>SANLPTVLVTGASGRTGQIVYKKLKEGSDKFVAKGLVRSAQGKEKIGGEADVFIGDITDADSINPAFQGIDA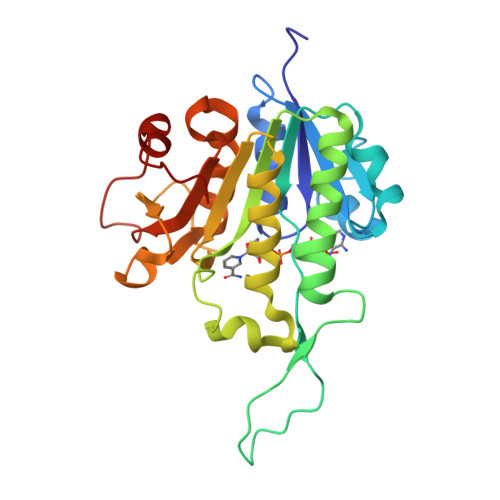LVILTSAVPKMKPGFDPTKGGRPEFIFEDGQYPEQVDWIGQKNQIDAAKVAGVKHIVVVGSMGGTNPDHPLNKLGNGNILVWKRKAEQYLADSGTPYTIIRAGGLLDKEGGVRELLVGKDDELLQTDTKTVPRADVAEVCIQALLFEEAKNKAFDLGSKPEGTSTPTKDFKALFSQVTSRF[2x]> GSHMASMHTVLQIGAGGVGSVVAHKMGMNRDVFKNIILASRSLDKCYAIKESMLKKGLGEIGVEQVDADDTQALVALIQKYKPKVVINVALPYQDLTIMQACLETKTHYIDTANYEHPDLAK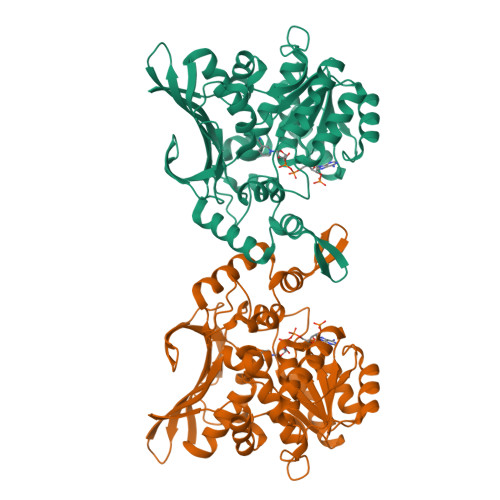FEYKEQWAFDRAYKEARILGVLGAGFDPGVTNAYVAHAQRHHFDTIHTLDILDCNAGDHKRPFATNFNPEINLREVSSKGRYYENGKWIETKPLEIKQVWAYPQIGEMDSYLLYHEELESLVKNIKGLRRARFFMTFSQNYLTHMKCLENVGMLGIKEIEHQGVKIVPIQFLKTLLPDPATLAKDTTGKTNIGCYMTGIKNNQDKTLYIYNVCDHKKCYEEVGSQAISYTTGVPAMCAAKMICNDTWSADHFRAGVFNIEELNTDPFMEELIKQGLPYEVIER> MLTEGISIQSYDGHTFGALVGSPAKAPAPVIVIAHEILGVNAFMRETVSWLVDQGYAAVCPDLHARQAPGTALDPQDEAQREQAYKLWQAFDMEAGVGDLEAAIRYARHLPYSNGKVGLVGYSLGGALAFLVAAKGCVDRAVGYCGVGLEKQLDKVPEVKHPALFHM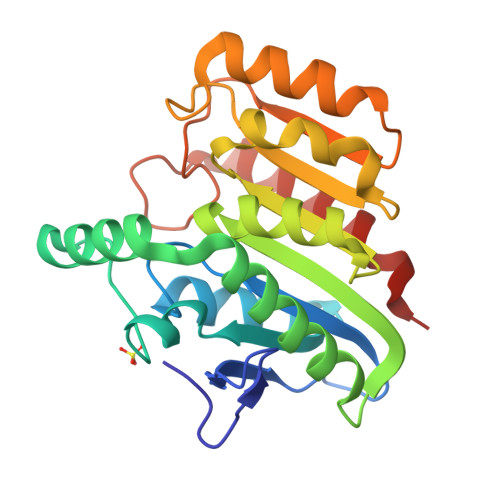GGQDHFVPAPSRQLITEGFGANPLLQVHWYEGAGHSFARTGSSDYVASAAALANERTLDFLAPLQSKKP>MSIVNILSVNVLNNPAKFSDPYKFEITFECLEPLKSDLEWKLTYVGSATSQSYDQILDTLLVGPIPIGINKFVFEADPPNIDLLPQLSDVLGVTVILLSCAYEDNEFVRVGYYVNNEMEGLNLQEMDDAEIKKVKVDISKVWRSILAEKPR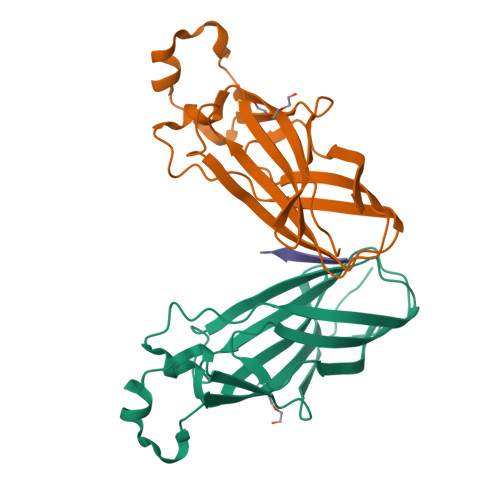VTRFNIQWDN[2x];> KDMQLARRLR 Imipenem 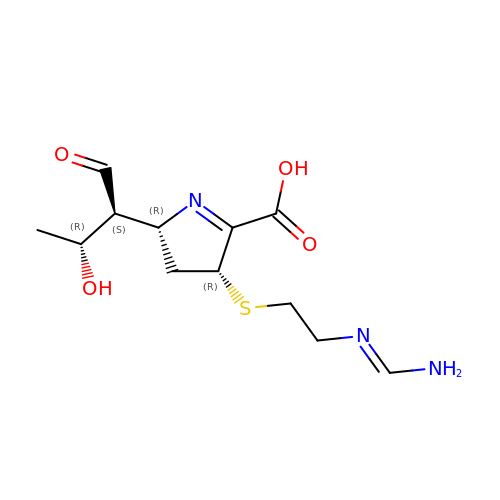| C12 H19 N3 O4 S | NIJGFQHESQFJAG-ZYUZMQFOSA-N>MIEKQMDRVVKEMRRQLEMIDKLTTREIEQVELLKRIHD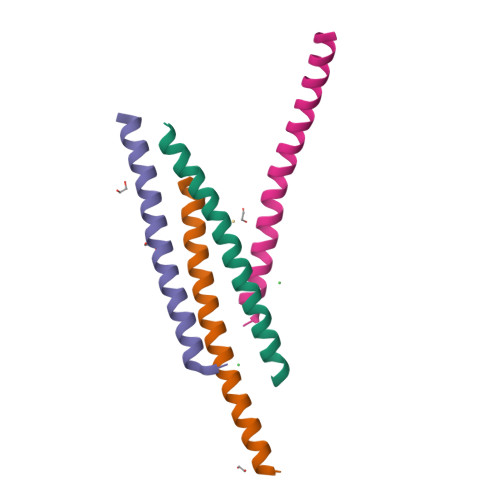KLVVQST[4x]>[2x]GSDYIIKEKTVLLQKKDSEGFGFVLRGAKAQTPIEEF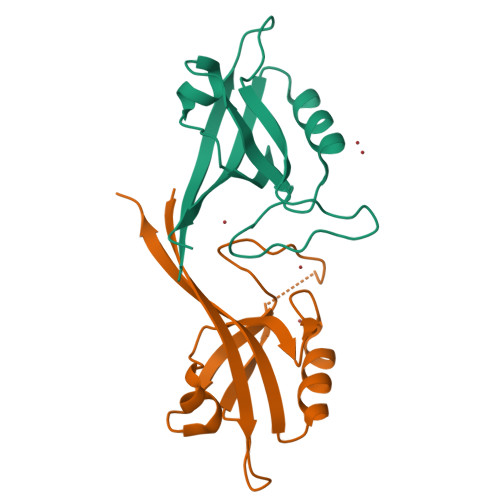TPTPAFPALQYLESVDEGGVAWRAGLRMGDFLIEVNGQNVVKVGHRQVVNMIRQGGNTLMVKVVMVTRHPDM> CYGGFDLYFILDKSGSVLHHWNEIYYFVEQLAHKFISPQLRMSFIVFSTRGTTLMKLTEDREQIRQGLEELQKVLPGGDTYMHEGFERASEQIYYENRQGYRTA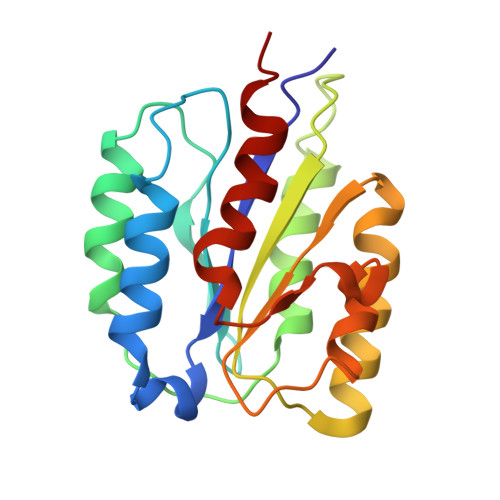SVIIALTDGELHEDLFFYSEREANRSRDLGAIVYAVGVKDFNETQLARIADSKDHVFPVNDGFQALQGIIHSILKKSC>[2x]HHHHHHASENLYFQGAMASEKHFKYVILGGGVAAGYAAREFAKQGVKPGELAIISKEAVAPYERPALSKGYLFPQNAARLPGFHVCVGSGGERLLPEWYSEKGIELILSTEIVKADLASKTLTSAVGATFTYEILIIATGSSVIKLSDFGTQGADSNNILY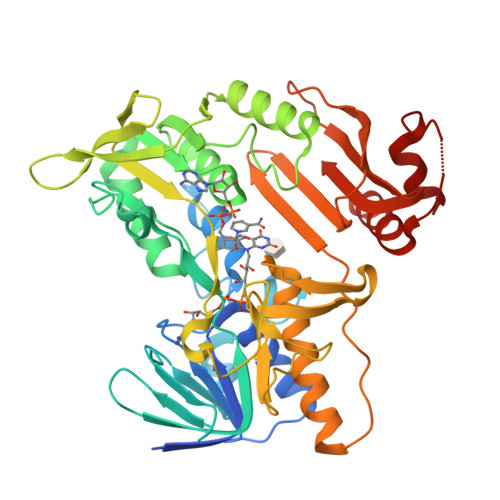LREVDDADKLVAAIQAKKGGKAVIVGGGYIGLELSAALKINDFDVTMVFPEPWCMPRLFTADIAAFYESYYTNKGVKIVKGTVAVGFDADANGDVTAVNLKNGSVLEADIVVVGVGGRPLTTLFKGQVAEEKGGIKTDAFFETSVPGVYAVGDVATFPMKMYNELRRVEHVDHARKSAEQAVKAIKGKESGESVVEYDYLPYFFSRSFDLGWQFYGDNVGDTILFGDSDPTSAKPKFGSYWIKDGKVLGAFLEGGSPDENKAIAKVAKTQPPVANIEELKKEGLQFASKI>MVILGVGYFLLGLILLYYGSDWFVLGSER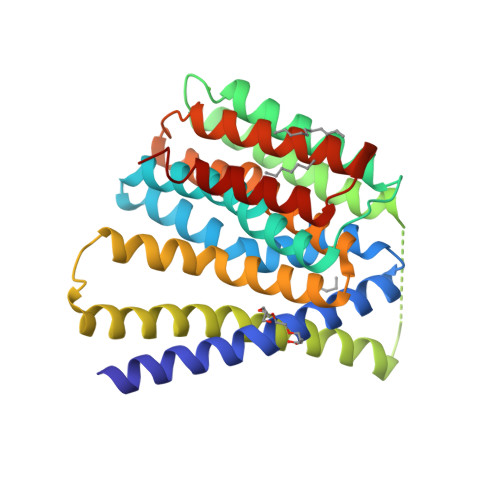IARHFNVSNFVIGATVMAIGTSLPEILTSAYASYMHAPGISIGNAIGSCICNIGLVLGLSAIISPIIVDKNLQKNILVYLLFVIFAAVIGIDGFSWIDGVVLLILFIIYLRWTVKNGSAEIEENNDKNNPSVVFSLVLLIIGLIGVLVGAELFVDGAKKIALALDISDKVIGFTLVAFGTSLPELMVSLAAAKRNLGGMVLGNVIGSNIADIGGALAVGSLFMHLPAENVQMAVLVIMSLLLYLFAKYSKIGRWQGILFLALYIIAIASLR[2x]> XVTIDADLM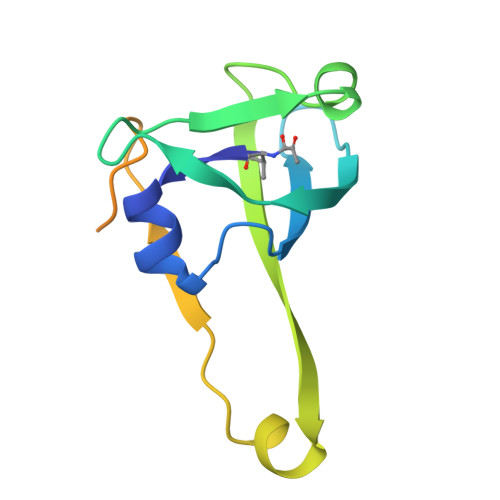DAADLLEGEQVTIVDIDNGARLVTYAITGERGSGVIGINGAAAHLVHPGDLVILIAYATMDDARARTYQPRIVFVDAYNKPIDMGHDPAFVPENAGELLDPRLGVGLEHHHHHH>[2x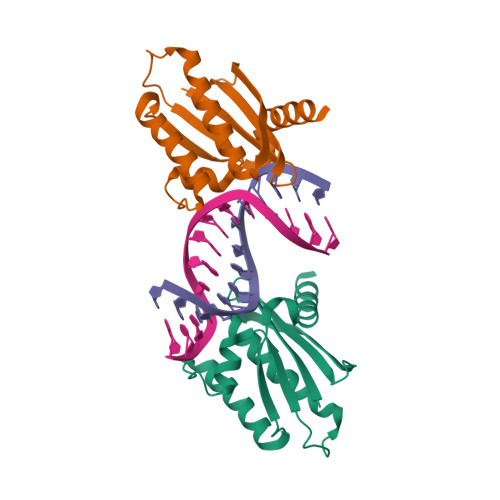]MNKIIIYTDGGARGNPGPAGIGVVITDEKGNTLHESSAYIGETTNNVAEYEALIRALEDLQMFGDKLVDMEVEVRMNSELIVRQMQGVYKVKEPTLKEKFAKIAHIKMERVPNLVFVHIPREKNARADELVNEAIDKALS>[4x]SMPPIFLPPPNYLFVRDVWKSNLYSEFAVIRQLVSQYNHVSISTEFVGTLARPIGTFRSKVDYHYQTMRANVDFLNPIQLGLSLSDANGNKPDNGPSTWQFNFEFDPKKEIMSTESLELLRKSGINFEKHENLGIDVFEFSQLLMDSGLMMDDSVTWITYHAAYDLGFLINILMNDSMPNNKEDFEWWVHQYMPNFYDLNLVYKIIQEFKNPQLQQSSQQQQQQQYSLTTLADELGLPRFSIFTTTGGQSLLMLLSFCQLSKLSMHKFPNGTDFAKYQGVIYGIDGDQ;>[4x]RSMSRPVQEMIPLKFFAVDEVSCQINQEGAPKDVVEKVLFVLNNVTLANLNNKVDELKKSLTPNYFSWFSTYLVTQRAKTEPNYHDLYSKVIVAMGSGLLHQFMVNVTLRQLFVLLSTKDEQAIDKKHLKNLASWLGCITLALNKPIKHKNIAFREMLIEAYKENRLEIVVPFVTKILQRASESKIFKPPNPWTVGIL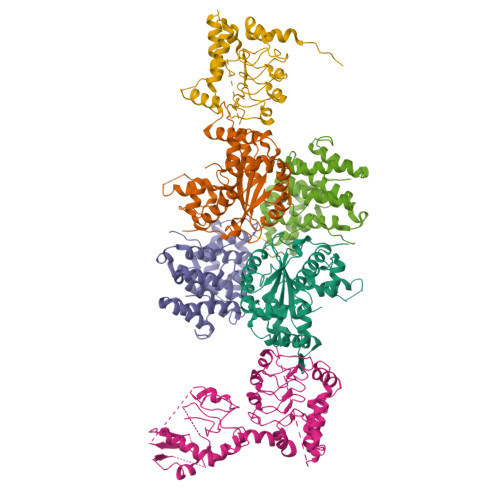KLLIELNEKANWKLSLTFEVEVLLKSFNLTTKSLKPSNFINTPEVIETLSG;>[4x]MNASTAAVNSIGMVPTVGTPVNINVNASNPLLHPHLDDPSLLNNPIWKLQLHLAAVSAQSLGQPNIYARQNAMKKYLATQQAQQAQQQAQQQAQQQVPGPFGPGPQAAPPALQPTDFQQSHIAEASKSLVDCTKQALMEMADTLTDSKTAKKQQPTGDSTPSGTATNSAVSTPLTPKIELFANGKDEANQALLQHKKLSQYSIDEDDDIENRMVMPKDSKYDDQLWHALDLSNLQIFNISANIFKYDFLTRLYLNGNSLTELPAEIKNLSNLRVLDLSHNRLTSLPAELGSCFQLKYFYFFDNMVTTLPWEFGNLCNLQFLGVEGNPLEKQFLKILTEKSVTGLIFYLRDNRPEIPLPHERRFIEINTDGEPQREYDSLQQSTEHLATDLAKRTFTVLSYNTLCQHYATPKMYRYTPSWALSWDYRRNKLKEQILSYDSDLLCLQEVESKTFEEYWVPLLDKHGYTGIFHAKARAKTMHSKDSKKVDGCCIFFKRDQFKLITKDAMDFSGAWMKHKKFQRTEDYLNRAMNKDNVALFLKLQHIPSGDTIWAVTTHLHWDPKFNDVKTFQVGVLLDHLETLLKEETSHNFRQDIKKFPVLICGDFNSYINSAVYELINTGRVQIHQEGNGRDFGYMSEKNFSHNLALKSSYNCIGELPFTNFTPSFTDVIDYIWFSTHALRVRGLLGEVDPEYVSKFIGFPNDKFPSDHIPLLARFEFMKTNTGSKKV> MSNKEKQMNLLSDKNVAIIGGGPVGLTMAKLLQQNGIDVSVYERDNDREARIFGGTLDLHKGSGQEAMKKAGLLQTYYDLALPMGVNIADEKGNILSTKNVKPENRFDNPEINRNDLRAILLNSLENDTVIWDRKLVMLEPGKKKWTLTFENKPSETADLVIIANGGMS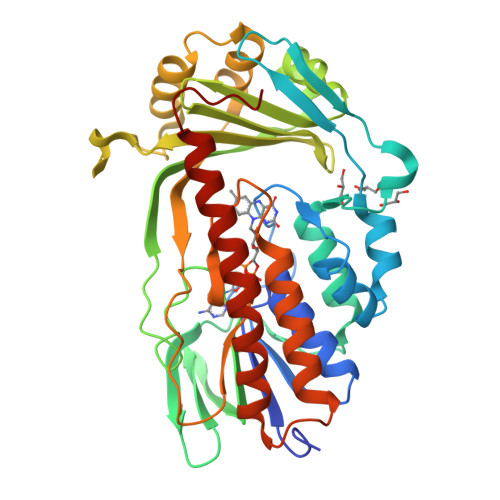KVRKFVTDTEVEETGTFNIQADIHHPEVNCPGFFQLCNGNRLMAAHQGNLLFANPNNNGALHFGISFKTPDEWKNQTQVDFQNRNSVVDFLLKEFSDWDERYKELIRVTSSFVGLATRIFPLGKSWKSKRPLPITMIGDAAHLMPPFAGQGVNSGLMDALILSDNLTNGKFNSIEEAIENYEQQMFIYGKEAQEESTQNEIEMFKPDFTFQQLLNV> MHHHHHHSSGRENLYFQGMGRRRAPELYRAPFPLYALQVDPSTGLLIAAGGGGAAKTGIKNGVHFLQLELINGRLSASLLHSHDTETRATMNLALAGDILAAGQDAHCQLLRFQAHQQQGNKAEKAGSKEQGPRQRKGAAPAEKKCGAETQHEGLELRVENLQAVQTDFSSDPLQKVVCFNHDNTLLATGGTDGYVRVWKVPSLEKVLEFKAHEGEIEDLALGPDGKLVTVGRDLKASVWQKDQLVTQLHWQENGPTFSSTPYRYQACRFGQVPDQPAGLRLFTVQIPHKRL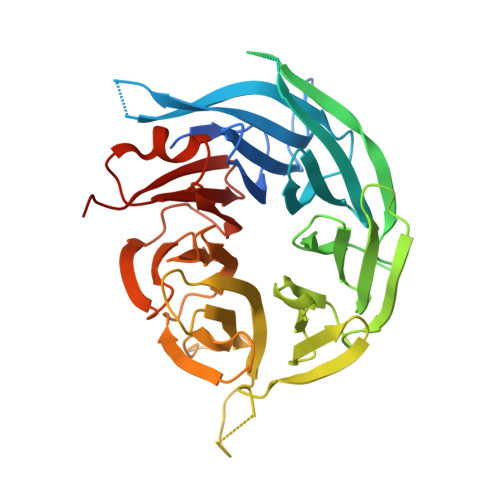RQPPPCYLTAWDGSNFLPLRTKSCGHEVVSCLDVSESGTFLGLGTVTGSVAIYIAFSLQCLYYVREAHGIVVTDVAFLPEKGRGPELLGSHETALFSVAVDSRCQLHLLPSRRSV>[2x]GSLEMAEPQAESEPAAGGARGGGGDWPAGLTTYRSIQVGPGAAARWDLCIDQAVVFIEDAIQYRSINHRVDASSMWLYRRYYSNVCQRTLSFTIFLILFLAFIETPSSLTSTADVRYRAAPWEPPCGLTESVEVLCLLVFAADLSVKGYLFGWAHFQKNLWLLGYLVVLVVSLVDWTVSLSLVCHEPLRIRRLLRPFFLLQNSSMMKKTLKCIRWSLPEMASVGLLLAIHLCLFTMFGMLLFAGGKQDDGQDRERLTYFQNLPESLTSLLVLLTTANNPDVMIPAYSKNRAYAIFFIVFTVIGSLFLMNLLTAIIYSQFRGYLMKSLQTSLFRRRLGTRAAFEVLSSMVGEGGAFPQAVGVKPQNLLQVLQKVQLDSSHKQAMMEKVRSYGSVLLSAEEFQKLFNELDRSVVKEHPPRPEYQSPFLQSAQFLFGHYYFDYLGNLIALANLVSICVFLVLDADVLPAERDDFILGILNCVFIVYYLLEMLLKVFALGLRGYLSYPSNVFDGLLTVVLLVLEISTLAVYRLPHPGWRPEMVGLLSLWDMTRMLNMLIVFRFLRIIPSMKPMAVVASTVLGLVQNMRAFGGILVVVYYVFAIIGINLFRGVIVALPGNSSLAPANGSAPCGSFEQLEYWANNFDDFAAALVTLWNLMVVNNWQVFLDAYRRYSGPWSKIYFVLWWLVSSVIWVNLFLALILENFLHKWDPRSHLQPLAGTPEATYQMTVELLFRDILEEPEEDELTERLSQHPHLWLCR

Two-pore channels (TPCs) belong to the voltage-gated ion channel superfamily and function as a homodimer, with each subunit containing two homologous Shaker-like 6-TM repeats. However, several recent studies have demonstrated that mammalian TPCs are sodium-selective channels activated by the endolysosome specific lipid phosphatidylinositol 3,5-bisphosphate (PI(3,5)P2) rather than NAADP. Like other TPC channels, HsTPC2 functions as a dimer with each subunit containing two homologous six-transmembrane domains (6-TM I and 6-TM II). Here we present the cryo-EM structures of human TPC2 (HsTPC2) in both the ligand-bound and apo states, which reveal the structural basis of phospholipid binding as well as its activation mechanism.

Interestingly, the single particles of HsTPC2 in the presence of PI(3,5)P2 can be partitioned into two classes of particles, and 3D refinement yielded HsTPC2 structures in the open and closed conformations at 3.7 Å and 3.4 Å resolution, respectively. The 3:5 ratio of the particles between the open and closed conformations in the PI(3,5)P2-bound structure of HsTPC2 likely represents the ligand efficacy of channel activation. The HsTPC2 ion conduction pore adopts both closed and open conformations in the ligand-bound state. In the open state, these constriction-forming residues dilate and rotate away from the central axis, resulting in a much wider opening at the intracellular gate. In the closed state, the IS6 helix breaks into two halves at Gly317, just below the cytosolic gate, while in the open state, IS6 becomes a long continuous helix. Upon ligand binding, the Arg329 side chain adopts an extended configuration to form salt bridges with the PI(3,5)P2 phosphate groups; this interaction provides an outward force to pull the IS6 helix into the straight conformation; meanwhile, Ser322 forms a hydrogen bond with the C5-phosphate of PI(3,5)P2 to help stabilize the IS6 helix in the open conformation. In the ligand-bound, closed state, Arg329 forms a salt bridge with the C3-phosphate, while in the ligand-bound open form, Arg329 forms salt bridges with both the C3- and C5-phosphates as well as a hydrogen bond with the C4 hydroxyl group; additionally, Ser322 forms a hydrogen bond with the C5-phosphate only in the open conformation. Between the two IS6 residues that interact with PI(3,5)P2 in the open state, Arg329 appears to play the determinant role in channel gating as its mutation (Arg329Ala) almost completely abolishes channel activity whereas the Ser322Ala mutation reduces the channel activity to a lesser extent. The movement of IS6 from the closed to open state results in the outward dilation and rotation of gating residues (Tyr312 and Thr308) at the bundle crossing. Interestingly, we also observed two long stretches of density plugging the open gate in the open HsTPC2 structure.(3E)-3-(1H-pyrrol-3-ylmethylidene)-3,4,5,6-tetrahydro-2,3'-bipyridine | C15 H15 N3 | 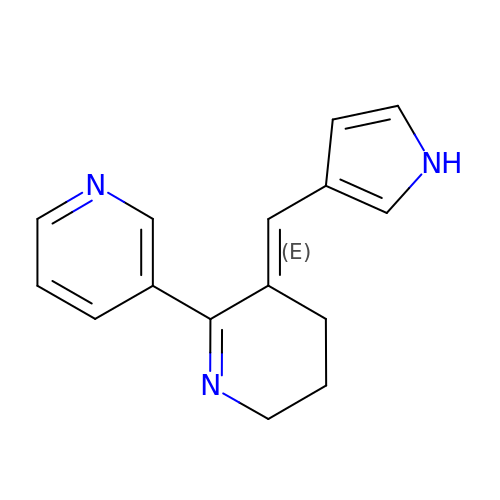LCDAAPCYCXHGRV-UKTHLTGXSA-N>[2x]GHMNDALHIGLPPFLVQANNEPRVLAAPEARMGYVLELVRANIAADGGPFAAAVFERDSGLLIAAGTNRVVPGRCSAAHAAILALSLAQAKLDTH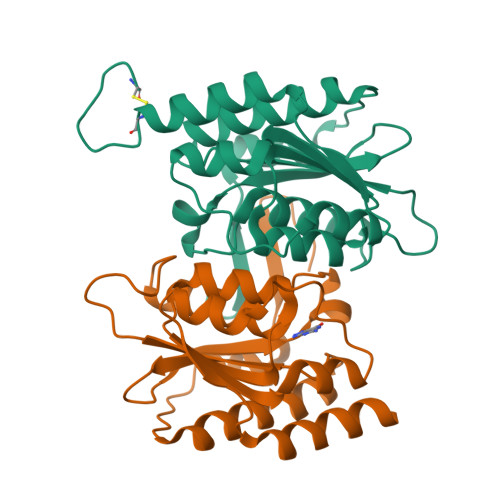DLSADGLPACELVTSAEPCVMCFGAVIWSGVRSLVCAARSDDVEAIGFDEGPRPENWMGGLEARGITVTTGLLRDAACALLREYNACNGVIYNARCGVHKGS> GSPGISGGGGGILDSMVEKLGKLQYSLDYDFQNNQLLVGIIQAAELP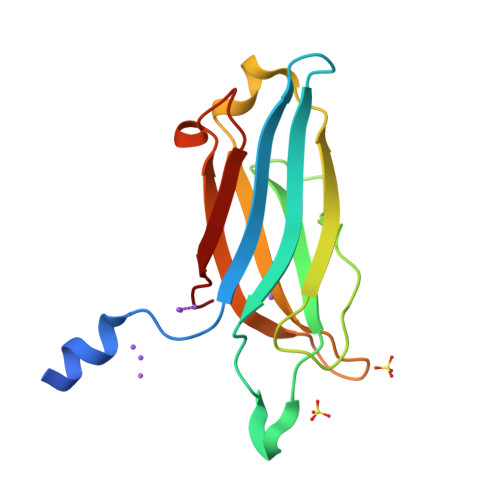ALDMGGTSDPYVKVFLLPDKKKKFETKVHRKTLNPVFNEQFTFKVPYSELGGKTLVMAVYDFDRFSKHDIIGEFKVPMNTVDFGHVTEEWRDLQSAE>[6x]MGGSTKLEEHLEGIVNIFHQYS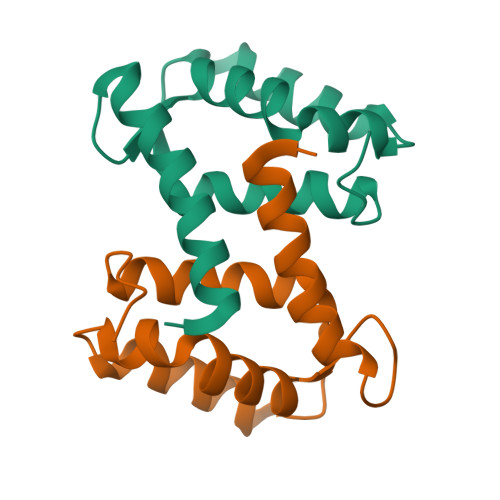VRKGHFDTLSKGELKQLLTKELANTIKNIKDKAVIDEIFQGLDANQDEQVDFQEFISLVAIALKAAHYHTHKE S. scabies produces a 200-residue, 22-kDa protein that is a single-domain enzyme called Scabin. Scabin has been cloned, expressed, and purified, and shown to harbor dual enzymatic activities (GH and ADP-ribosyltransferase). Scabin targets DNA as a substrate for ADP-ribose modification; it also shows enzyme specificity towards genomic DNA from Solanum tuberosum tubers. Scabin shares nearly 40% sequence identity with the Pierisin family of mARTs.

According to our Scabin-NAD+-DNA model, Tyr129 is important for binding DNA, based on its location and orientation in the complex. Our model suggests that Tyr129 reaches into the DNA minor groove and contacts both the DNA I and II strands. Previously, Tyr129 was shown to be important for DNA binding, but was not involved in the reaction mechanism. However, binding of DNA substrate is likely controlled by a rather large contact area and contributions from several backbone and side-chains within the Scabin active site. Several replacements at Tyr129 were made to ascertain the chemical nature of the Scabin-DNA interaction. Trp128 and Tyr129 interact with adjacent nucleotides to the guanine nucleophile, allowing Trp155 to dock to the target guanine base. The rest of the Scabin variants showed either a WT-like crystal structure or similar CD spectra to the WT in solution. All the structures were of high quality, ranging from 1.5 to 1.75 Å.

> MGSSHHHHHHSSGENLYFQGSHMTATATSAKAAAPACPRFDDPVHAAADPRVDVERITPDPVWRTTCGTLYRSDSRGPAVVFEQGFLPKDVIDGQYDIESYVLVNQPSPYVSTTYDHDLYKTWHKSGYNYYIDAPGGVDVNKTIGDRHKWADQVEVAFPGGIRTEFVIGVCPVDKKTRTEKMSECVGNPHYEPWH>GSMDSKHQCVKLNDGHFMPVLGFGTYAPPEVPRSKALEVTKLAIEAGFRHIDSAHLYNNEEQVGLAIRSKIADGSVKREDIFYTSKLWSTFHRPELVRPALENSLKKAQLDYVDLYLIHSPMSLKPGEELSPTDENGKVIFDIVDLCTTWEAMEKCKDAGLAKSIGVSNFNRRQLEMILNKPGLKYKPVCNQVECHPYFNRSKLLDFCKSKDIVLVAYSALGSQ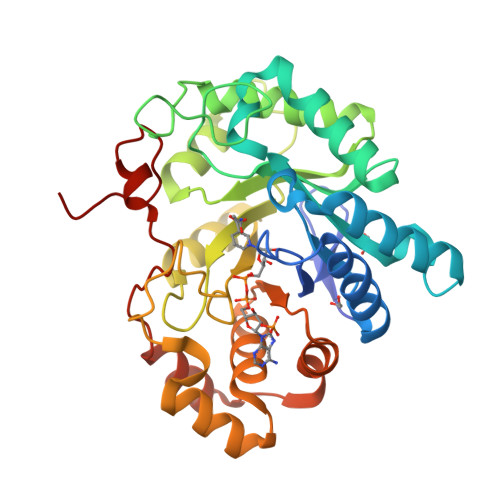RDKRWVDPNSPVLLEDPVLCALAKKHKRTPALIALRYQLQRGVVVLAKSYNEQRIRQNVQVFEFQLTAEDMKAIDGLDRNLHYFNSDSFASHPNYPYSDEY[2x]2-azanyl-3-methyl-benzoic acid | C8 H9 N O2 | 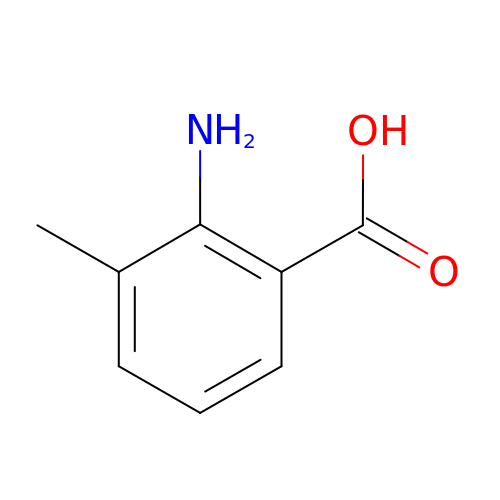WNAJXPYVTFYEST-UHFFFAOYSA-N N-{[(3S)-1-acetylpiperidin-3-yl]methyl}methanesulfonamide | C9 H18 N2 O3 S | 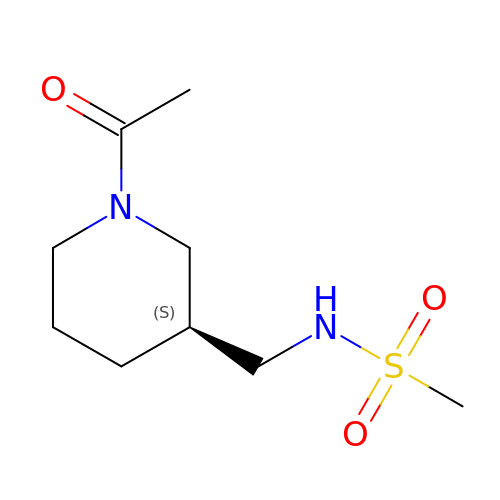CCRQXLDMMWNHIR-UHFFFAOYSA-N In Pseudomonas aeruginosa, an important opportunistic pathogen that causes numerous acute and chronic infections, the hybrid two-component system (TCS) regulates the swarming ability and biofilm formation with a multistep phospho­relay, and consists of hybrid-sensor histidine kinase (HK), histidine-containing phospho­transfer protein (Hpt) and response regulator (RR). HptB, the target protein in this work, is closely related to biofilm formation, which could increase drug resistance and protect the cell from pinocytosis by the host. According to previous studies, after the sensor proteins PA1611, PA1976 and PA2824 are auto­phospho­rylated, the phospho­ryl group is transferred to HptB and subsequently to the downstream RR protein PA3346 as illustrated in Fig. 1. In this work, two crystal structures of HptB and the receiver domain of HK PA1611 (PA1611REC) of P. aeruginosa have been determined in order to elucidate their interactions for the transfer of the phospho­ryl group. The HptB–PA1611REC complex is further modeled to analyze the binding surface and interactions between the two proteins.

Then, we successfully crystallized the native HptB in another tetragonal space group, P43212, with six protein molecules in one asymmetric unit. The crystal structure of native HptB was subsequently determined with the mutant HptB structure as an initial model and refined to high resolution (1.58 Å). The structural differences between mutant and native HptB are small, with an RMSD of 0.15 Å. The structures of six native HptBs in one asymmetric unit are essentially the same, with a small RMSD of 0.16 Å overall for the Cα atoms [Fig. 3(b)]. The structure of HptB comprises five α-helices and folds into an elongated α-helical bundle with an up-and-down topology. The helices α2 (Tyr22–Gln45), α3 (Ala49–Asn65), α4 (Val69–Arg83) and α5 (Ala90–Arg112) are twisted around the central axis and form an antiparallel four-helix bundle. Residues Ala46–Asp48, Met66–Ala68 and Arg84–Arg89 form short turns between helices α2–α3, α3–α4 and α4–α5, respectively. The four-helix bundle is covered with the short N-terminal helix α1 (Asp8–Met18) which protrudes into the solvent environment and connects to helix α2 with a 310 helix (Glu19–Glu21) [Fig. 3(c)]. In HptB, this conserved histidine residue, His57, is located near the middle of helix α3. The imidazole side chain of His57 protrudes from the bundle and is exposed to solvent [Figs. 3(c) and 3(d)]. The hydrogen-bonding linkages between Lys60 and Glu79 prohibit their side chains from shielding the imidazole ring of the active-site histidine. High solvent accessibility of the imidazole ring is achieved through the nearby small side-chain volume, which results from the highly conserved glycine residue (Gly61 in HptB) at position +4 from the active-site histidine.

>MSAPHLDDRVLASLQEVMEDEYPVLLDTFVLDSEERLRSLHAALQAGDAQALRHTAHSFKGGSSNMGAVLLAGYCKELEESARRGELQRAPALIEQMEREFAIVRILFKQERQRYR[6x]>GHMSHWIWQHKDWPHFFWDEKLLSSHLSSARLVQGKLLGIIHTINQQTARQMNAFVLADQAVDTSAIEGEHLNRDSVRSSIANRLGLKQVGINKPVDRYIEGLLDMLLDATENYEQPLTLERLYGWHAALFPTGYSGIHKITVAALRKTDPMQIVSGRPGKIKVHYEAPPSKRVNKEMRIFLNWFNKKDLDGLLRAGIAHLWFELLHPFDDGNGRIGRAIIDLTLAQDEKQNVRYYSLSSAIMQDRKNYYTQLGKSCRGNMDITLWLIWFINCFKTAIHQAFELIDDITLKSRFWEKHATTELNARQIKVLNRLLDAGKKGFIGGMTTRKYTQLTKTSRTTAYRELHDLVLKKCLKPLTKKGRSAAYEIRWVNKEHKSKK[2x]

Here, we identify the protein product of CBU_0822, in the following referred to as Coxiella burnetii Fic enzyme 2 (CbFic2), as a DNA-binding protein and AMP-transferase that AMPylates Histone H3 at S10 and S28. We show that CbFic2 acts as a bifunctional enzyme, both capable of AMPylation as well as deAMPylation, and is regulated by the binding of DNA via a C-terminal helix-turn-helix domain. According to sequence analysis using SMART including outlier homologs and PFAM domains, it encompasses a conserved Fic domain (115–223 aa, Fic motif HPFDDGNGRIGR 205–216 aa) with N-terminal inhibitory helix (TSAIEG, 62–67 aa), an N-terminal domain of unknown function (DUF4172 domain, 4–85 aa) and a C-terminal helix-turn-helix (HTH) domain (304–362 aa) of the DeoR family. We propose that CbFic2 performs AMPylation in its monomeric state, switching to a deAMPylating dimer upon DNA binding.

In the asymmetric unit of the crystal, CbFic2 is present as a symmetrical homodimer which, according to the program PISA52, is the only probable assembly and is predicted to be stable. Within the dimer, the interface is composed of amino acids 20–43 aa in helix α1 within the N-terminal DUF4172 domain. According to an analysis by PDBsum53, residues S22 and S26 interact across the interface. The crystal structure reveals the predicted HTH domain to be a 2-stranded winged HTH domain where the tri-helical HTH motif is followed by a β-hairpin wing. PDBeFold55 analysis of the HTH domain of crystallized CbFic2 revealed structural similarity (Q-score >0.48) albeit low sequence similarity (%seq < 18%) to Z-DNA-binding (ZDB) proteins, which belong to the same subclass of wHTH domains as proteins of the DeoR family. A structural superimposition of CbFic2’s HTH domain with the B-DNA-binding human transcription factor E2F4 and the Z-DNA-binding domain hZαADAR1 of human double-stranded RNA-specific adenosine deaminase ADAR1 reveals that this tyrosine is not present at the conserved position in CbFic2, but moved by one helix turn toward the N-terminus (Y341), similar to the tyrosine in E2F4 but with a different rotation. Looking at the dimerization interface of CbFic2’s crystal structure, high salt conditions would destroy the polar and electrostatic interaction as well as the hydrogen bonds involved in the interface. At first glance, superposition of the CbFic2 structure with crystallized HTH domains in complex with DNA makes dimer formation of CbFic2 via the crystal dimer interface unlikely to be compatible with a simultaneous binding of both HTH domains to the same DNA-strand of about 20 bp, if not for a major rearrangement of CbFic2 or bending of DNA. However, AlphaFold prediction of CbFic2 results in five models, which show flexibility in the orientation of the HTH domain in relation to the Fic and DUF domain, communicated by a kink in the long connecting helix between the HTH and Fic domains.> ASIPSSASVQLDSYNYDGSTFSGKIYVKNIAYSKKVTVVYADGSDNWNNNGNIIAASFSGPISGSNYEYWTFSASVKGIKEFYIKYEVS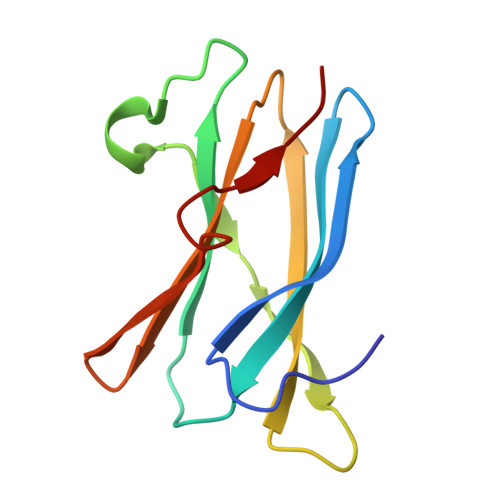GKTYYDNNNSANYQVST> MDPIINGNSANVYLTDSYLKGVISFSECNALGSYIFNGPYLKNDYTNLISRQNPLIEHMNLKKLNITQSLISKYHKGEIKLEEPTYFQSLLMTYKSMTSSEQIATTNLLKKIIRRAIEISDVKVYAILNKLGLKEKDKIKSNNGQDEDNSVITTIIKDDILSAVKDNQSHLKADKNHSTKQKDTIKTTLLKKLMCSMQHPPSWLIHWFNLYTKLNNILTQYRSNEVKNHGFTLIDNQTLSGFQFILNQYGCIVYHKELKRITVTTYNQFLTWKDISLSRLNVCLITWISNCLNTLNKSLGLRCGFNNVILTQLFLYGDCILKLFHNEGFYIIKEVEGFIMSLILNITEEDQFRKRFYNSMLNNITDAANKAQKNLLSRVCHTLLDKTVSDNIINGRWIILLSKFLKLIKLAGDNNLNNLSELYFLFRIFGHPMVDERQAMDAVKINCNETKFYLLSSLSMLRGAFIYRIIKGFVNNYNRWPTLRNAIVLPLRWLTYYKLNTYPSLLELTERDLIVLSGLRFYREFRLPKKVDLEMIINDKAISPPKNLIWTSFPRNYMPSHIQNYIEHEKLKFSESDKSRRVLEYYLRDNKFNECDLYNCVVNQSYLNNPNHVVSLTGKERELSVGRMFAMQPGMFRQVQILAEKMIAENILQFFPESLTRYGDLELQKILELKAGISNKSNRYNDNYNNYISKCSIITDLSKFNQAFRYETSCICSDVLDELHGVQSLFSWLHLTIPHVTIICTYRHAPPYIGDHIVDLNNVDEQSGLYRYHMGGIEGWCQKLWTIEAISLLDLISLKGKFSITALINGDNQSIDISKPIRLMEGQTHAQADYLLALNSLKLLYKEYAGIGHKLKGTETYISRDMQFMSKTIQHNGVYYPASIKKVLRVGPWINTILDDFKVSLESIGSLTQELEYRGESLLCSLIFRNVWLYNQIALQLKNHALCNNKLYLDILKVLKHLKTFFNLDNIDTALTLYMNLPMLFGGGDPNLLYRSFYRRTPDFLTEAIVHSVFILSYYTNHDLKDKLQDLSDDRLNKFLTCIITFDKNPNAEFVTLMRDPQALGSERQAKITSEINRLAVTEVLSTAPNKIFSKSAQHYTTTEIDLNDIMQNIEPTYPHGLRVVYESLPFYKAEKIVNLISGTKSITNILEKTSAIDLTDIDRATEMMRKNITLLIRILPLDCNRDKREILSMENLSITELSKYVRERSWSLSNIVGVTSPSIMYTMDIKYTTSTISSGIIIEKYNVNSLTRGERGPTKPWVGSSTQEKKTMPVYNRQVLTKKQRDQIDLLAKLDWVYASIDNKDEFMEELSIGTLGLTYEKAKKLFPQYLSVNYLHRLTVSSRPCEFPASIPAYRTTNYHFDTSPINRILTEKYGDEDIDIVFQNCISFGLSLMSVVEQFTNVCPNRIILIPKLNEIHLMKPPIFTGDVDIHKLKQVIQKQHMFLPDKISLTQYVELFLSNKTLKSGSHVNSNLILAHKISDYFHNTYILSTNLAGHWILIIQLMKDSKGIFEKDWGEGYITDHMFINLKVFFNAYKTYLLCFHKGYGKAKLECDMNTSDLLCVLELIDSSYWKSMSKVFLEQKVIKYILSQDASLHRVKGCHSFKLWFLKRLNVAEFTVCPWVVNIDYHPTHMKAILTYIDLVRMGLINIDRIHIKNKHKFNDEFYTSNLFYINYNFSDNTHLLTKHIRIANSELENNYNKLYHPTPETLENILANPIK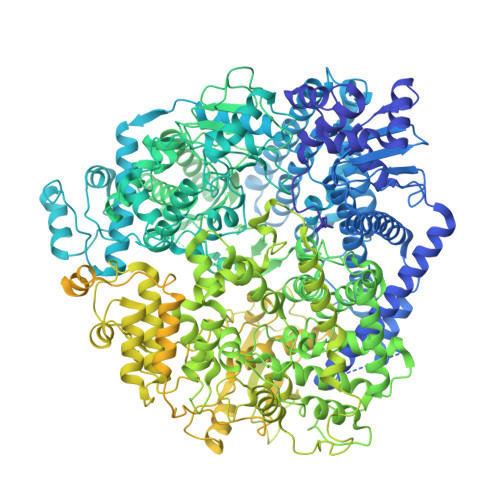SNDKKTLNDYCIGKNVDSIMLPLLSNKKLIKSSAMIRTNYSKQDLYNLFPMVVIDRIIDHSGNTAKSNQLYTTTSHQISLVHNSTSLYCMLPWHHINRFNFVFSSTGCKISIEYILKDLKIKDPNCIAFIGEGAGNLLLRTVVELHPDIRYIYRSLKDCNDHSLPIEFLRLYNGHINIDYGENLTIPATDATNNIHWSYLHIKFAEPISLFVCDAELSVTVNWSKIIIEWSKHVRKCKYCSSVNKCMLIVKYHAQDDIDFKLDNITILKTYVCLGSKLKGSEVYLVLTIGPANIFPVFNVVQNAKLILSRTKNFIMPKKADKESIDANIKSLIPFLCYPITKKGINTALSKLKSVVSGDILSYSIAGRNEVFSNKLINHKHMNILKWFNHVLNFRSTELNYNHLYMVESTYPYLSELLNSLTTNELKKLIKITGSLLYNFHNE> SLEARAALNQALEMKRQGKREKAQKLFMHALKMDPDFVDALTEFGIFSEEDKDI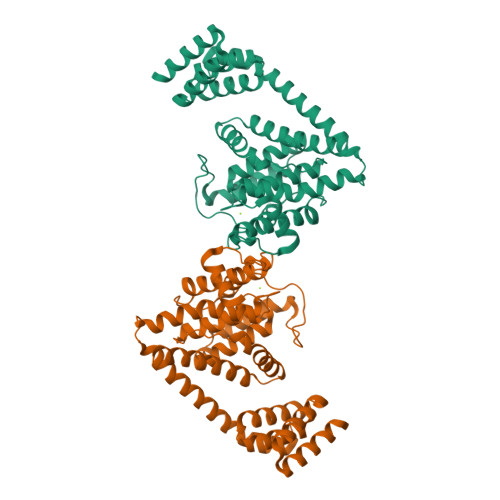IQADYLYTRALTISPYHEKALVNRDRTLPLVEEIDQRYFSIIDSKVKKVMSIPKGNSALRRVMEETYYHHIYHTVAIEGNTLTLSEIRHILETRYAVPGSSLEEQNEVIGMHAAMKYINTTLVSRIGSVTISDVLEIHRRVLGYVDPVEAGRFRTTQVLVGHHIPPHPQDVEKQMQEFVQWLNSEEAMNLHPVEFAALAHYKLVYIHPFIDGNGRTSRLLMNLILMQAGYPPITIRKEQRSDYYHVLEAANEGDVRPFIRFIAKCTETTLDTLLFATTEYSVALPEAQP> MLNSFKLSLQYILPKLWLTRLAGWGASKRAGWLTKLVIDLFVKYYKVDMKEAQKPDTASYRTFNEFFVRPLRDEVRPIDTDPNVLVM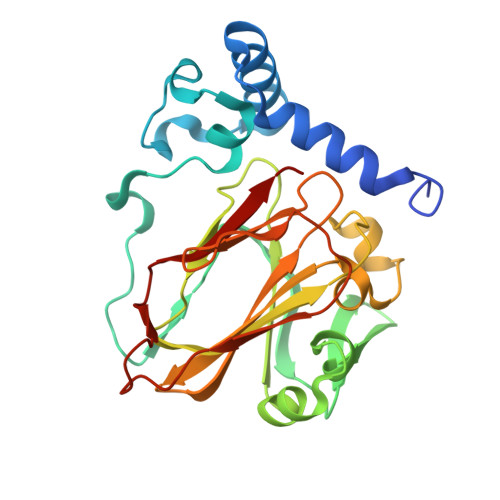PADGVISQLGKIEEDKILQAKGHNYSLEALLAGNYLMADLFRNGTFVTTYLSPRDYHRVHMPCNGILREMIYVPGDLFSVNHLTAQNVPNLFARNERVICLFDTEFGPMAQILVGATIVGSIETVWAGTITPPREGIIKRWTWPAGENDGSVALLKGQEMGRFKLG>[2x]MAAGESMAQRMVWVDLEMTGLDIEKDQIIEMACLITDSDLNILAEGPNLIIKQPDELLDSMSDWCKEHHGKSGLTKAVKESTITLQQAEYEFLSFVRQQTPPGLCPLAGNSVHEDKKFLDKYMPQFMKHLHYRIIDVSTVKELCRRWYPEEYEFAPKKAASHRALDAISESIKELQFYRNNIFKKK

Human RNA exoribonuclease 2 (Rexo2) is an evolutionarily conserved 3′-to-5′ DEDDh-family exonuclease located primarily in mitochondria. Rexo2 degrades small RNA oligonucleotides of <5 nucleotides (nanoRNA) in a way similar to Escherichia coli Oligoribonuclease (ORN), suggesting that it plays a role in RNA turnover in mitochondria. Rexo2 forms a homodimer and interacts mainly with the last two 3′-end nucleobases of substrates by hydrophobic and π−π stacking interactions via Leu53, Trp96, and Tyr164, signifying its preference in binding and degrading short oligonucleotides without sequence specificity. Rexo2 contains four strictly conserved DEDD residues (D47, E49, D147, D199) for binding two metal ions, as well as a general base (H194) in the active site for hydrolysis of the phosphodiester bonds in nucleic acid substrates.

We obtained three complex cocrystals, referred to as Rexo2–RNA (Rexo2–D199A bound with a 12-nt U12 RNA and Mg2+), Rexo2–DNA1 (wild-type Rexo2 bound with a 5-nt T5 DNA), and Rexo2-DNA2 (Rexo2–D199A bound with a 10-nt T10 DNA and Mg2+). In the Rexo2–RNA complex, we used the inactive D199A mutant for cocrystallization with RNA in the presence of Mg2+. D199 is one of the metal-ion binding residues in the DEDDh active site, but we still identified two Mg2+ ions in the active site, one bound to Glu49 (A site, MgA) and another bound to Asp47 and Asp147 (B site, MgB). However, several regions in protomer A were disordered, including residues 51–59, 85–114, and 190–193, in the Rexo2–RNA structure. As a result, the RNA substrate was modeled only in the active site of protomer B, but not modeled in protomer A due to the ill-defined electron density. In the Rexo2–RNA and Rexo2–DNA1 complexes, only the last two 3′-end nucleotides were observed, i.e., U–U in Rexo2–RNA and T–T in Rexo2–DNA1, with the remainder of the substrates being disordered. RNA-specific interactions are observed in the Rexo2–RNA complex, where the 2′-OH (O2′) of the ribose group of the 3′-end nucleotide forms a hydrogen bond with the Met50 backbone (O atom). This interaction likely facilitates product release for nucleoside monophosphates, so RNA is cleaved more efficiently than DNA. We propose a hydrolysis mechanism for Rexo2 activity, based on comparison of the structures of the two active sites in the Rexo2–RNA and Rexo2–DNA1 complexes. Thus, Rexo2 hydrolyzes the phosphodiester linkage from the 3′-OH end by means of a two-Mg2+-ion-dependent catalytic mechanism.> MKGLRKSILCLVLSAGVIAPVTSGMIQSPQKCYAYSINQKAYSNTYQEFTNIDQAKAWGNAQYKKYGL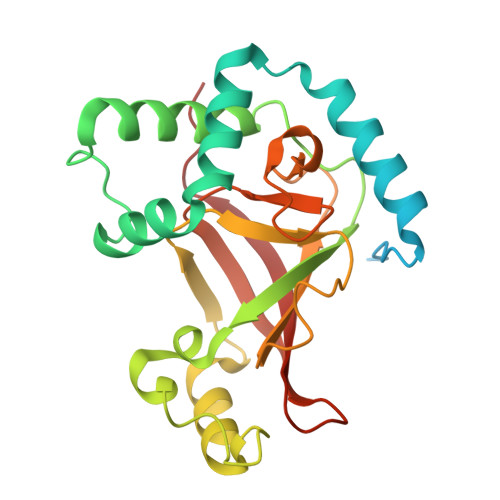SKSEKEAIVSYTKSASEINGKLRQNKGVINGFPSNLIKQVELLDKSFNKMKTPENIMLFRGDDPAYLGTEFQNTLLNSNGTINKTAFEKAKAKFLNKDRLEYGYISTSLMNVSQFAGRPIITKFKVAKGSKAGYIDPISAFAGQLEMLLPRHSTYHIDDMRLSSDGKQIIITATMMGTAINPK>VCSCRLVFCRRTELRVGNCLIGGVSFAYCCT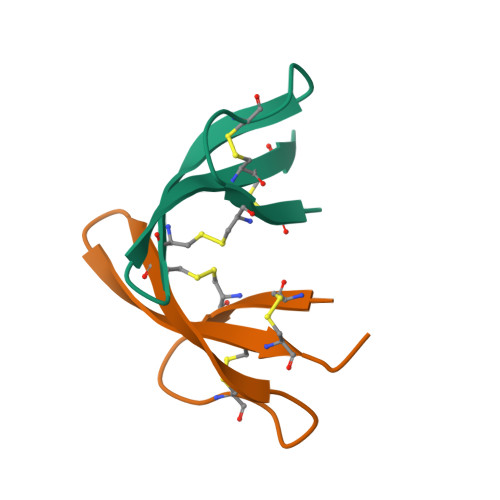RV[8x]> LQRTTLRCYSALVGQ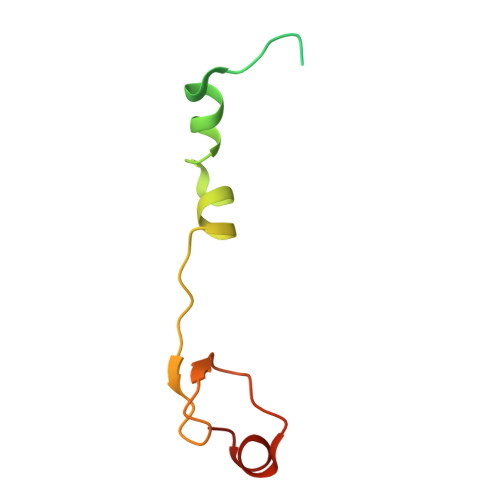ATPVLLGSKGGTPKRKKNPMQLRRKTYGLHFKERYLKLEEWYFCPLCAEPKKQGEWCRREDCRQIKP> MNPSQTQKGKIQIQVSRGSIDLLVRTMYEDINNIKLKNERFQKKKRAEDERRRRERYAEIQQEAIASGKKNAALEMKWAELKELDECEELNREMQDQQQTFQQIIEGKENLRKEFEEELKRKDDEYVKMLKEQSNDIKDMISKMRSQFYKIRDANMQELEDIERHFEQERSNLLNEFKAKIQATFKKHLDLEEQYVKEHAKTEEEQTKNIEDLRIKGAKHYAELKITMETEIQDLEKCFEDMKALYQLITEKLDYSLKVLQEKFHENNSMCDELKRKENNFKNRLKQLTKDYKQYDKKFKLENKNLTQEYKRIIRQFKELQKKFKHFEKADLDKYSEIQKMNEAEVKELKDKIIKCNITIHIQQLGMQWIPPQSEEEILAQQKLQLEQGGKAEEEEEREFEFCISEIKIGEICNIILEE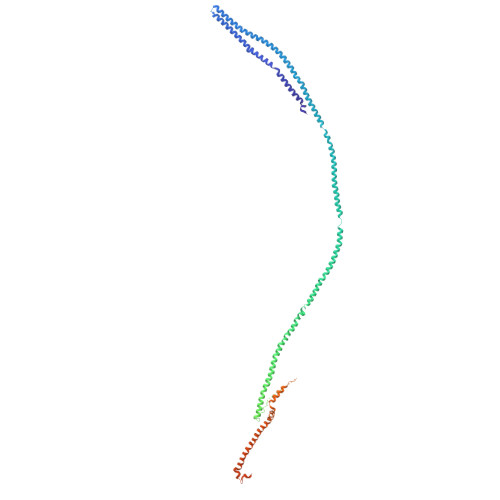ADFLIDDKLREELEGSAEPEQIFQRLDCIKKCLYIDSEDEMNLFFRELITKCRVKSAEEIEEEARKQLLLLGLIKEAEENENPEGEEVQQQEGAQQKKKEEGNKKDDPKGKEGAKDSKENANPQGQNKSNQDERKKKKDGQDDHAGQGQGQYDSNQGGMGENQEEGENAEGQENLEGEIEKEIDLENTQINLNEVVKFLQNWQANKDKRKEKLEKESSKKAVKQETEREKKERIAREGKKYWEKLTQVLPERTFRIWNVNFFKFSFEKQILLNQINKLRFWTDLCPNIMNFFWTDKNQSKKPVNCITKMKNQRIFQINTYKLIMNLLSALQDSLIQIKDKDDFIQTKISTNLFTFHNFQILLQIFIVNQSFLFIRLCQSYSKKIILLIKNINQKLFNLSNFKNQFSF> MVYQVKDQEDFTKQLNEAG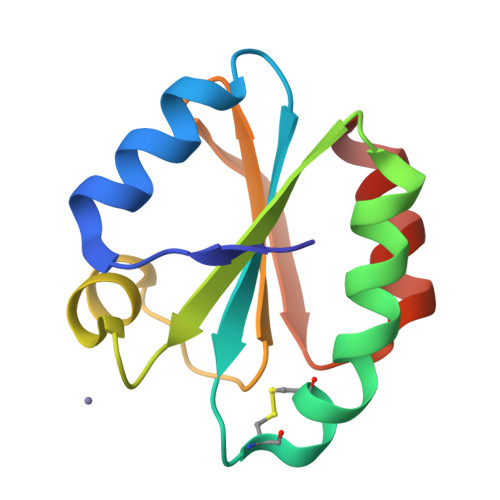NKLVVIDFYATWCGPCKMIAPKLEELSQSMSDVVFLKVDVDECEDIAQDNQIASMPTFLFMKNGQKLDSLSGANYDKLLELVEKNK> GSMSEEQVAQDTEEVFRSYVFYRHQQEQEAEGVAAPADPEMVTLPLQPSSTMGQVGRQLAIIGDDINRRYDSEFQTMLQHLQPTAENAYEYFTKIATSLFESGINWGRVVAL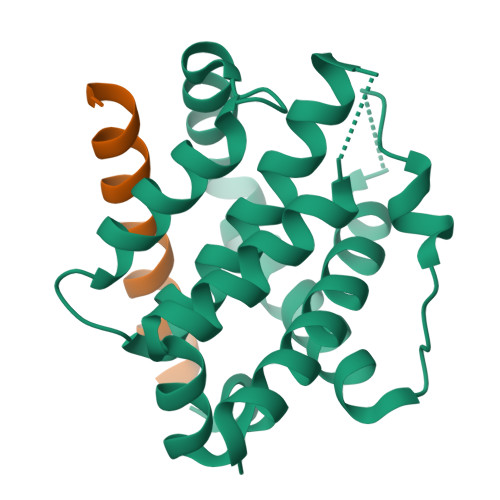LGFGYRLALHVYQHGLTGFLGQVTRFVVDFMLHHSIARWIAQRGGWVAALNL;> DAIIQMIVELLKRVGDQWEEEQSLAS We have determined high-resolution crystal structures of the ykkC guanidine III riboswitch from Thermobifida fusca. X-ray crystallography shows that the RNA folds into an H-type pseudoknot, in which a connecting strand locates in the major groove of one duplex to form a regular triple helix. This continues into the central core of conserved nucleotides that form a novel left-handed helical ramp of inter-nucleotide interactions, generating the guanidinium cation binding site. Comparison with earlier probing data suggest that the formation of the triple helix is stabilized by guanidine binding and this exposes the adjacent ribosome binding site to permit initiation of gene translation.

Using in-line probing experiments, Sherlock and Breaker (2017) showed that methylguanidine and aminoguanidine bound to the riboswitch with only a small loss of affinity, suggesting that the additional methyl and amino groups could be accommodated in this space. Methylguanidine and aminoguanidine were co-crystallized with the riboswitch RNA, while ethylguanidine and agmatine were soaked into ligand-free crystals. All crystallized in the trigonal space group P3121, and all diffracted to good resolution (2.01–2.32 Å). The structures were solved by SAD using the bromine atoms. Methylguanidine, aminoguanidine, and ethylguanidine were each bound in the same way as guanidine. Each nitrogen atom was hydrogen bonded to G7, G17, and C6 in the same manner as unmodified guanidine, with the additional methyl, amino, or ethyl groups attached to the nitrogen hydrogen bonded to G17 N7. The appended side chains were co-planar with the guanidine atoms, and directed laterally through the side opening. Like the guanidine II riboswitch (Huang et al., 2017), we present here structures with methyl-, ethyl-, and aminoguanidine bound, showing that the additional alkyl and amino groups are tolerated within the structure. These occupy the position taken by an ordered water molecule in the structure with bound guanidine. The side opening can accommodate a range of small side chains, with affinities in the order guanidine > methylguanidine ∼ aminoguanidine > ethylguanidine > agmatine.

>CCGGACGAGGUGCGCCGUACCCGGUCAGGACAAGACGGCGC[2x]> MGSSHHHHHHSSGHIEGRHGEEQPPETAAQRCFCQVSGYL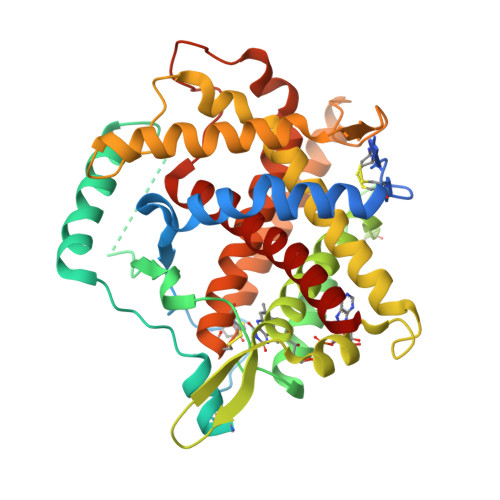DDCTCDVETIDRFNNYRLFPRLQKLLESDYFRYYKVNLKRPCPFWNDISQCGRRDAAVKPAQSDEVPDGIKSASYKYSEEANNLIEECEQAERLGAVDESLSEETQKAVLQWTKHDDSSDNFAEADDIQSPEAEYVDLLLNPERYTGYKGPDAWKIWNVIYEENCFKPQTIKRPLNPLASGQGTSEENTFYSWLEGLCVEKRAFYRLISGLHASINVHLSARYLLQETWLEKKWGHNITEFQQRFDGILTEGEGPRRLKNLYFLYLIELRALSKVLPFFERPDFQLFTGNKIQDEENKMLLLEILHEIKSFPLHFDENSFFAGDKKEAHKLKEDFRLHFRNISRIMDCVGCFKCRLWGKLQTQGLGTALKILFSEKLIANMPESGPSYEFHLTRQEIVSLFNAFGRISTSVKELENFRNLLQNIH> AHHHERLRLRRDFLLIFKEGKSLQNEYFVVLFRKNGLDYSRLGIVVKRKFGKATRRNKLKRWVREIFRRNKGVIPKGFDIVVIPRKKL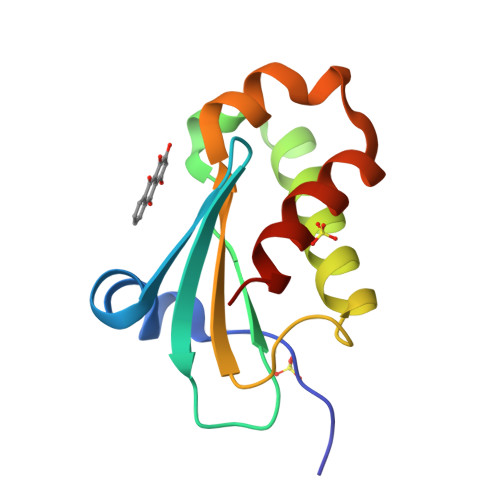SEEFERVDFWTVREKLLNLLKRIEG> SELSFNYPNFQSVEDITFQGGASPRNETLQLTPTDSNGIPIRQRAGHAVYSQPFQLRDTSFYTTFTFVIRTTSNSPADGFAIFIAPPDFPVKRYGGYLGLFEPNTATNTSANKVVAVEFDTWVNTEWKEPRYRHIGI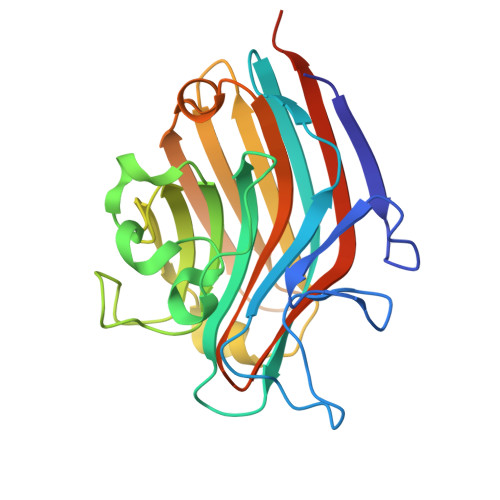DVNSIVSVRVTRWQDKDVFSRSIATAHVGYDGISKILTAFVTYPDGGNYVLSHVVDLAEIFPGDVRIGFSGATGQYETQYIHSWSFSSTSTNLLRDGARHHHHHH Proton-dependent oligopeptide transporters (POTs) belong to the major facilitator superfamily (MFS) and transport short-chain peptides from the extracellular environment into the target cell. Previously reported structures revealed that the bacterial POTs possess 14 helices, of which H1–H6 and H7–H12 constitute the typical MFS fold and the residual two helices, HA and HB, are inserted between H6 and H7. PepTSo2 from Shewanella oneidensis is a unique POT transporter that has been reported to assemble as a 200 kDa tetramer in the detergent-solubilized form. In this study, a combination of X-ray crystallographic and single-particle cryo-EM analyses revealed the species-specific tetramer formation mechanism of PepTSo2, in which the two asparagine residues in H12 and the unpreserved ECL play key roles.

Tetramer formation was confirmed by a single-particle analysis using cryo-EM and was further analyzed by X-ray crystallographic analyses using lipidic cubic phase (LCP) crystallization. Although square-shaped particles were clearly observed in the cryo-EM micrographs of PepTSo2 reconstructed in Salipro, the overall resolution was limited to 6.7 Å and the quality of the map was too poor to refine the atomic model owing to severe orientation bias. The difference in the lipids used for reconstruction in this study might affect the physical properties of the specimen under solution conditions and thus cause the preferred specimen-orientation problem. To alleviate the orientation bias, we tried to collect data by tilting the grid from 30° to 50°, which drastically improved the data quality. However, the atomic-level oligomerization mechanism remained unclear because of the resolution limit. In all of the structures determined in this study, each PepTSo2 protomer adopts a similar inward-open state, which might reflect cooperative substrate transport in the tetramer.

>[4x]MTLGTNQVSKTHSFMTVSLIELWERFGYYGMQALIVYFMVQRLGFDDSRANLVWSACAALIYVSPAIGGWVGDKILGTKRTMLLGAGILSVGYALMTVPTENTWFMFSALGVIVVGNGLFKPNAGNLVRKIYEGDDSKIDSAFTIYYMAVNVGSTFSMLLTPWIKDYVNAQYGNEFGWHAAFAVCCVGILVGLGNYALMHKSLANYGSEPDTRPVNKKSLAIVLALAALSVVASAIILEYEDVARVFVYAAGVAVLGIFFHLIRTSEPSERAGLIAALILTVQTVFFFIFYQQMSTSLALFALRNVDWDFQVFGTHLWTWSPAQFQALNPIWIMVLSPVLAWSYSWAGRNNKDFSIAAKFALGFAVVAIGFFIYGFAGQFAVNGKTSSWVMIWGYASYSLGELLVSGLGLAMIARYVPARMGGFMMGAYFVASGISQYLGGVVANFASVPQDLVDPLQTLPVYTNLFNKLGVAAVVCTIIALAVLPLMRRLTESHHAHSSIENNAAASLRDVKAEQLESSGENLYFQ>AMMRRGEIWQVDLDPARGSEANNQRPAVVVSNDRANATATRLGRGVITVVPVTSNIAKVYPFQVLLSATTTGLQVDCKAQAEQIRSIATERL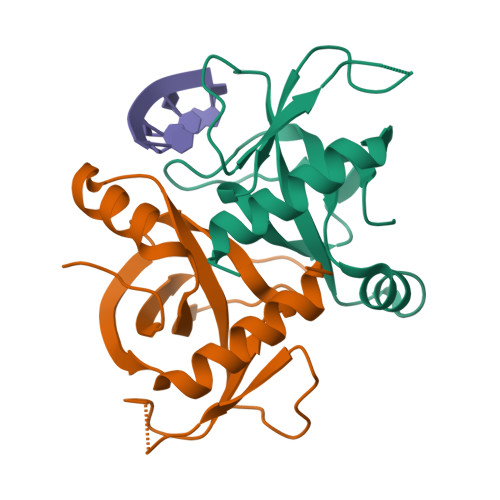LRPIGRVSAAELAQLDEALKLHLDLWS[2x]> MGPLWLDVAGYELSAEDREILQHPTVGGVILFGRNYHDNQQLLALNKAIRQAAKRPILIGVDQEGGRVQRFREGFSRIPPAQYYARAENGVELAEQGGWLMAAELIAHDVDLSFAPVLDMGFACKAIGNRAFGEDVQTVLKHSSAFLRGMKAVGMATTGKHFPGHGAVIADSHLETPYDERETIAQDMAIFRAQIEAGVLDAMMPAHVVYPHYDAQPASGSSYWLKQVLREELGFKGIVFSDDLSMEGAAVMGGPVER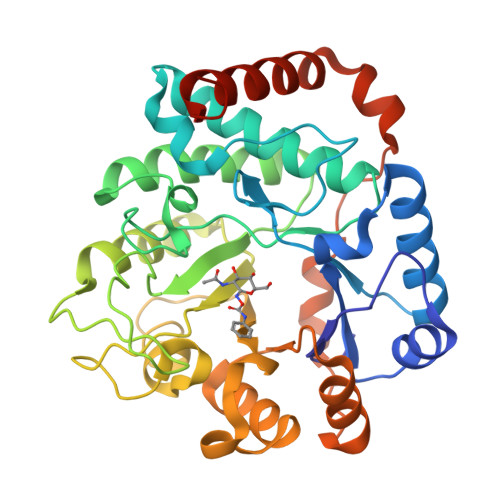SHQALVAGCDMILICNKREAAVEVLDNLPIMEVPQAEALLKKQQFSYSELKRLERWQQASANMQRLIEQFSEHHHHHHHHHH5-(2-thienyl)-1,3,4-thiadiazol-2-amine | C6 H5 N3 S2 | 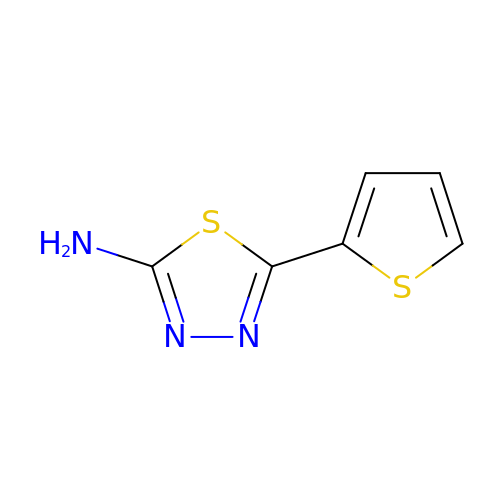DADKTCVAPDOGJQ-UHFFFAOYSA-N>[4x]MKYILVTGGVISGIGKGIIASSIGTILKSCGLRVTAIKIDPYINIDAGTFSPYEHGEVFVLNDGGEVDLDLGNYERFLDINLYKDNNITTGKIYQHVINKERRGDYLGKTVQVVPHITDAVQEWVMNQAKVPVDGNKEEPQICVIELGGTIGDIEGMPFVEAFRQFQFKAKRENFCNIHVSLVPQLSATGEQKTKPTQNSVRALRGLGLSPDLIVCRSSTPIEMAVKEKISMFCHVNPEQVICIHDVSSTYRVPVLLEEQSIVKYFKERLHLPIGDSASNLLFKWRNMADRYERLQKICSIALVGKYTKLRDCYASVFKALEHSALAINHKLNLMYIDSIDLEKITETEDPVKFHEAWQKLCKADGILVPGGFGIRGTLGKLQAISWARTKKIPFLGVCLGM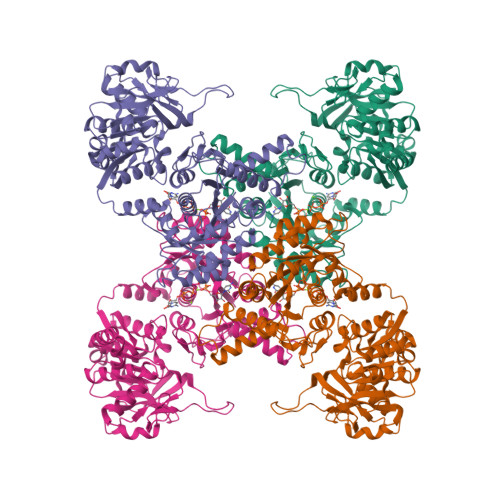QLAVIEFARNCLNLKDADSTEFRPNAPVPLVIDMPEHNPGNLGGTMRLGIRRTVFKTENSILRKLYGDVPFIEERHRHRFEVNPNLIKQFEQNDLSFVGQDVDGDRMEIIELANHPYFVGVQFHPEFSSRPMKPSPPYLGLLLAATGNLNAYLQQGCKLSSSDRYSDASDDSFSEPRIAELEIS> GADYDLKFGMVAGPSSNEYKAVEFFAKEVKEKSNGKIDVAIFPSSQLGDDRVMIKQLKDGALDFTLGESARFQIYFPEAEVFALPYMIPNFETSKKALLDTKFGQGLLKKIDKELNVQVLSVAYNGTRQTTSNRAINSIEDMKGLKLRVPNAATNLAYAKYVGAAPTPMAFSEVYLALQTNSVDGQENPLPTIQAQKFYEVQKYLALTNHILNDQLYLISNDTLADLPEDLQKVVKDAAAKAAEYHTKLFVDGENSLVEFFKSQGVTVTQPDLKPFKAALTPYYDEYLKKNGEVGKMAIEEISNLAKL

The first step of this process is the transport of sialic acid to the cytoplasm, which often takes place using a tripartite ATP-independent transport system consisting of a periplasmic binding protein and a membrane transporter. In this paper, the structural characterization of periplasmic binding proteins from the pathogenic bacteria Fusobacterium nucleatum, Pasteurella multocida and Vibrio cholerae and their thermodynamic characterization are reported. The structure and the thermodynamics of the binding of sugars suggest that all of these proteins have a very well conserved binding pocket and similar binding affinities. While the C1 carboxylate has been identified as the primary binding site, a second conserved hydrogen-bonding network is involved in the initiation and stabilization of the conformational states.

Pm-SiaP and Fn-SiaP were crystallized together with Neu5Ac. Their structures were determined to 1.57 and 2.5 Å resolution, respectively. The structure of Pm-SiaP was refined to an R factor of 0.17 and a free R factor of 0.20, and that of Fn-SiaP was refined to an R factor of 0.21 and a free R factor of 0.25. Superposition of the structures of the Neu5Ac-bound forms of the proteins resulted in an r.m.s. deviation of the 301 Cα atoms of between 0.4 and 0.6 Å. All three proteins (Pm-SiaP, Fn-SiaP and Hi-SiaP) have very similar structures, distinguished by two domains on either side of a well defined pocket, within which Neu5Ac binds. In all of the Neu5Ac-bound structures, a consistent pattern was seen in how Neu5Ac interacts with four of the residues within the pocket. Similar inter­actions between these four residues and Neu5Ac exist in Hi-SiaP and Pm-SiaP, with minor differences in sequence numbering (e.g. Arg127 and Arg147 are involved in the first two interactions in Hi-SiaP), as also seen previously. There was one interaction seen in Hi-SiaP (between Asn10 and O10 of Neu5Ac) that was not evident in Fn-SiaP and Pm-SiaP. The binding affinities of Fn-SiaP and Pm-SiaP to Neu5Ac are 45.5 and 19.7 nM, respectively. Thus, it was interesting that the SiaPs of F. nucleatum and P. multocida bound both forms of SA with equal affinity, and that there was only a moderate decrease in the binding of Neu5Gc in the case of V. cholerae.> MDLTNVSSLLNMERAR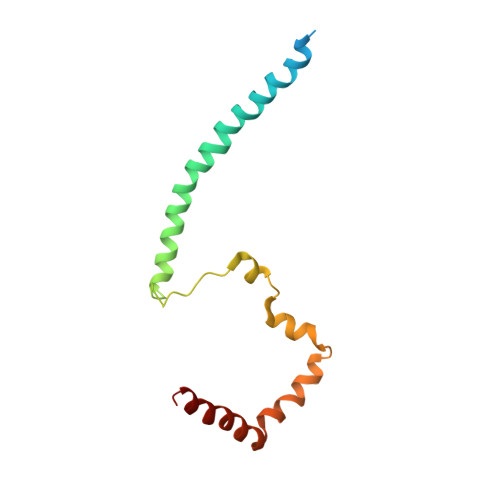DKANEEGLALLQEEIDKMVETTELMTGNIQSLKNKIQILASEVEEEEERVKQMHQINSSGVLSLPELSQKTLKAPTLQKEILALIPNQNALLKDLDILHNSSQMKSMSTFIEEAYKKLDAS> GMNSDIIVADFWKNNEEILTDFDKDSFCESWTENEMWSIEFKVAQTPKNAHCYSFLDYESSVYFRGQEFVVKQLSHDAVGKTLSKDIRAPHIYYTCQDGRQDDAITGSFTLEQCLTHIFKTDNRGFSWEIIDPSNILEKVQQENFGNNNYLTLI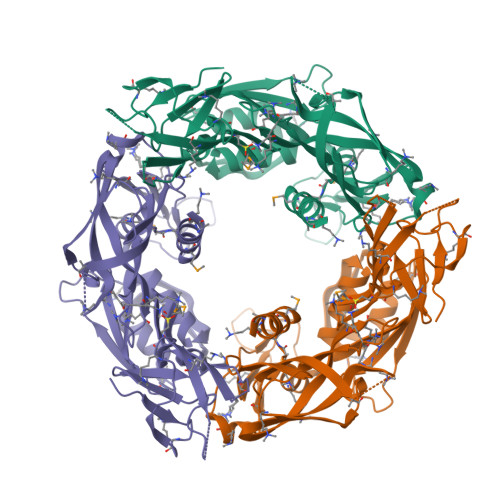DQLLDDYGVVVIPDNRHLVFKPREIYGAKTENFIRYKYNTDEASFDIDTLSLKTKIKGYGKVDSNGNNYFSPITYTSPEVEKWGIRWQEPVSDERYTVAGNMQRRLKLELQDYPATTGSVILKNDYECEKGDYVLFIYEPLGIDYDVQIVAYKKYPFTIKAPEITLSNNKKSIVSIMAQLAKVLKGAK> MHHHHH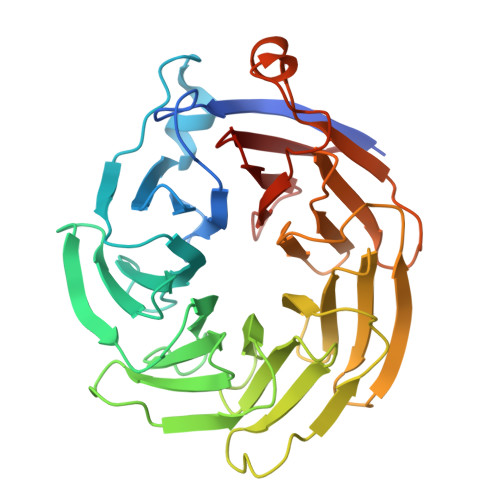HHHTFTRYSRLRVIAEIRHGDIFHSANIVSSIEFDRDDELFATAGVSRCIKVFDFSSVVNEPADMQCPIVEMSTRSKLSCLSWNKHEKNHIASSDYEGIVTVWDVTTRQSLMEYEEHEKRAWSVDFSRTEPSMLVSGSDDCKVKVWCTRQEASVINIDMKANICCVKYNPGSSNYIAVGSADHHIHYYDLRNISQPLHVFSGHKKAVSYVKFLSNNELASASTDSTLRLWDVKDNLPVRTFRGHTNEKNFVGLTVNSEYLACGSETNEVYVYHKEITRPVTSHRFGSPDMDDAEEEAGSYFISAVCWKSDSPTMLTANSQGTIKVLVLAA(2Z)-4,6-dihydroxy-2-[(8-methoxy-1,2,3,4-tetrahydropyrazino[1,2-a]indol-10-yl)methylidene]-1-benzofuran-3(2H)-one | C21 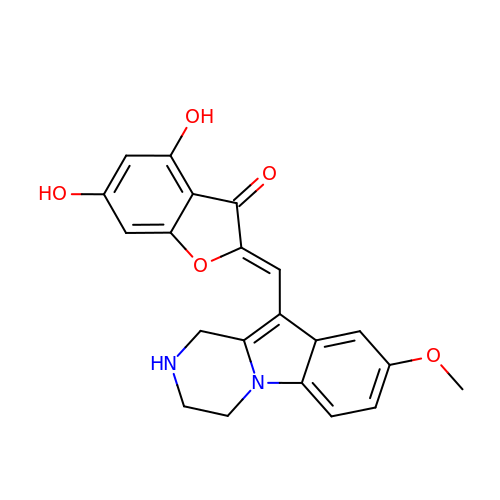H18 N2 O5 | HUEDLQSVQCSQPS-OCKHKDLRSA-N2,4,6,8,10,12-hexahydroxy-2lambda~5~,4lambda~5~,6lambda~5~,8lambda~5~,10lambda~5~,12lambda~5~-cyclohexaphosphoxane-2,4,6,8,10,12-hexone 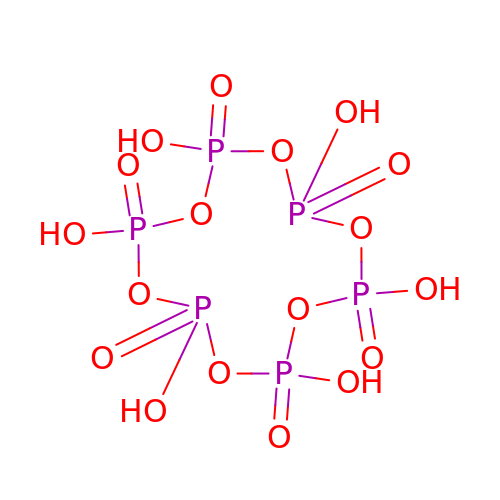| H6 O18 P6 | SZGVJLCXTSBVKL-UHFFFAOYSA-N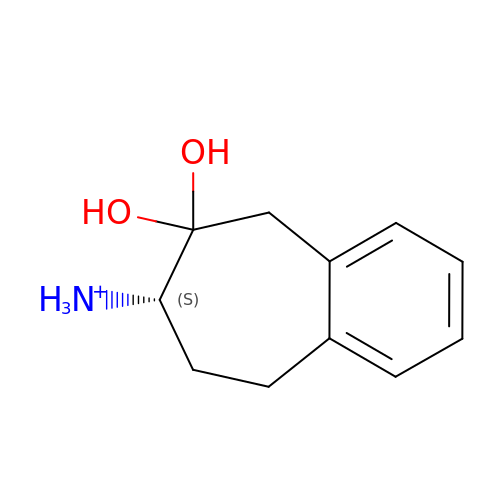[(7~{S})-6,6-bis(oxidanyl)-5,7,8,9-tetrahydrobenzo[7]annulen-7-yl]azanium | C11 H16 N O2 | DUYOIJVXOKTLQG-JTQLQIEISA-O> AMDGTAAEPRPGAGSLQHAQPPPQPRKKRPEDFKFGKILGEGSFSTVVLARELATSREYAIKILEKRHIIKENKVPYVTRERDVMSRLDHPFFVKLYFTFQDDEKLYFGLSYAKNGELLKYIRKIGSFDETCTRFYTAEIVSALEYLHGKGIIHRDLKPENILLNEDMHIQITDFGTAKVLSPESKQARANSFVGTAQYVSPELLTEKSACKSSDLWALGCIIYQLVAGLPPFRAGNEGLIFAKIIKLEYDFPEKFFPKARDLVEKLLVLDAT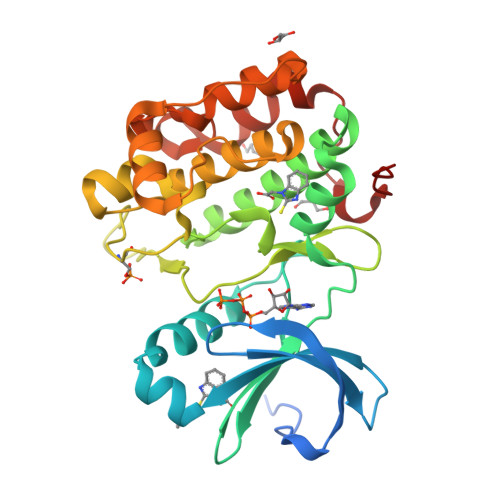KRLGCEEMEGYGPLKAHPFFESVTWENLHQQTPPKLT>SNAVNMMECITVSDVINVSVEEVWKKI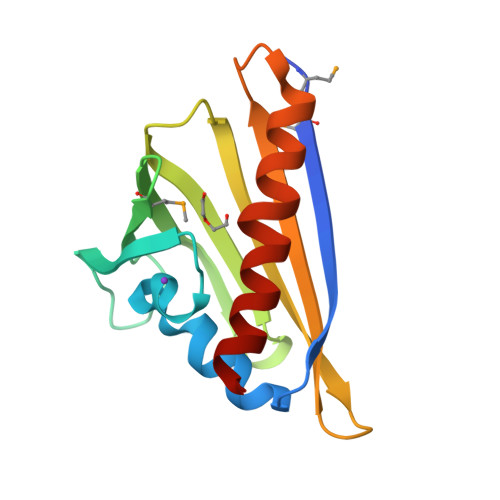SAFDEFSDYHPGAVRSFYLHQAADQQGSIRRVEMSDGYVEELLVNIDPKNYHLEYSILKSSFPLDGYSAEIKLIPVTQDNRTFIQWNVSFTTTHPSPEALVAEIKNNVLIAGINGLNDYFSKS[4x]>[2x]MAHHHHHHQPQKRKPKTGILMLNMGGPETLGDVHDFLLRLFLDRDLMTLPIQNKLAPFIAKRLTPKIQEQYRRIGGGSPIKIWTSKQGEGMVKLLDELSPNTAPHKYYIGFRYVHPLTEEAIEEMERDGLERAIAFTQYPQYSCSTTGSSLNAIYRYYNQVGRKPTMKWSTIDRWPTHHLLIQCFADHILKELDHFPLEKRSEVVILFSAHSLPMSVVNRGDPYPQEVSATVQKVMERL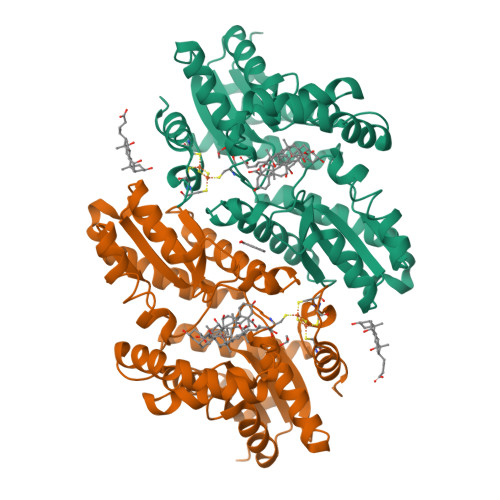EYCNPYRLVWQSKVGPMPWLGPQTDESIKGLCERGRKNILLVPIAFTSDHIETLYELDIEYSQVLAKECGVENIRRAESLNGNPLFSKALADLVHSHIQSNELCSKQLTLSCPLCVNPVCRETKSFFTSQQL> MDDPVAGDQLKSIVERIERLEEEKKTIADDIKEVYAEAKGNGYDVKVMRKVIAMRKRDANERAEEEAILDLYMQA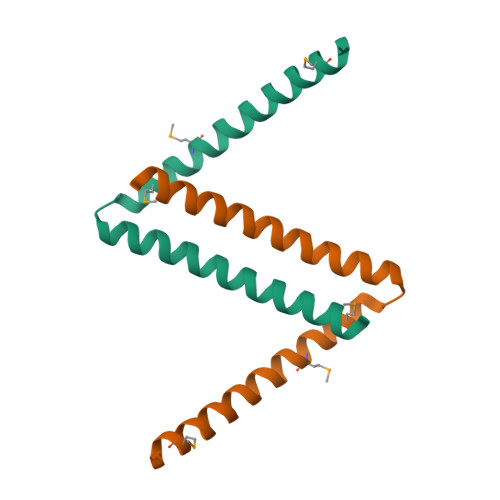VGESA>[4x]MASWKGLIHQYKEFLPVTDQTPALTLHEGNTPLIHLPKLSEQLGIELHVKTEGVNPTGSFKDRGMVMAVAKAKEEGNDTIMCASTGNTSAAAAAYAARANMKCIVI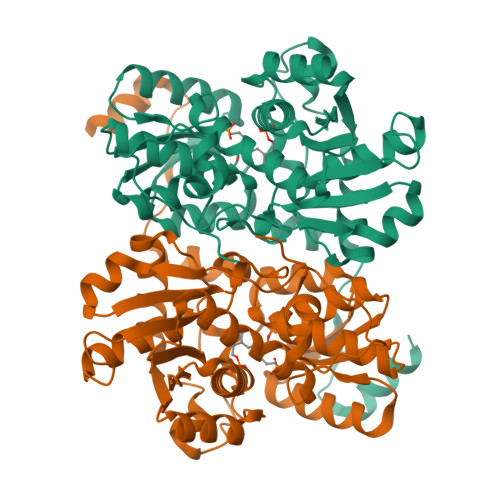IPNGKIAFGKLAQAVMYGAEIIAIDGNFDDALKIVRSICEKSPIALVNSVNPYRLEGQKTAAFEVCEQLGEAPDVLAIPVGNAGNISAYWKGFKEYHEKNGTSLPKMRGFEAEGSAAIVRNEVIENPETIATAIRIGNPASWDKAVKAAEESNGKIDEVTDDEILHAYQLIAREEGVFAEPGSCASIAGVLKQVKSGEIPKGSKVVAVLTGNGLKDPNTAVDISEIKPVTLPTNEDSILEYVKGAARV(3R)-3-{3-[(4-fluorophenyl)methyl]-1,2,4-oxadiazol-5-yl}-N-hydroxyheptanamide 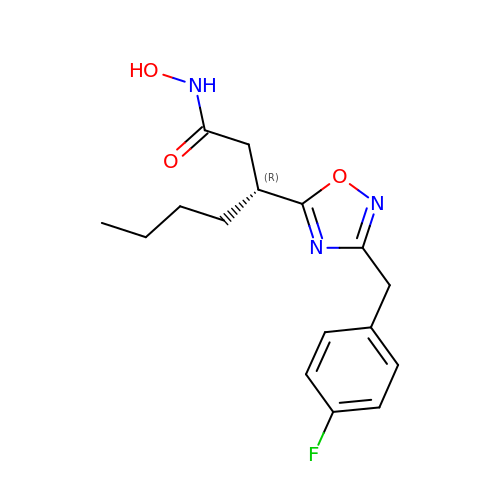| C16 H20 F N3 O3 | NPHICFLHFQUZKX-GFCCVEGCSA-N> MERLWKDIKRDWLLYAMLLPTIIWFLIFLYKPMIGLQMAFKQYSAWKGIAGSPWIGFDHFVTLFQSEQFIRAIKNTLTLSGLSLLFGFPMPILLALMINEVYSKGYRKAVQTIVYLPHFISIVIVAGLVVTFLSPSTGVVNNMLSWIGLDRVYFLTQPEWFRPIYISSNIWKEAGFDSIVYLAAIMSINPALYESAQVDGATRWQMITRITLPCIVPTIAVLLVIRLGHILE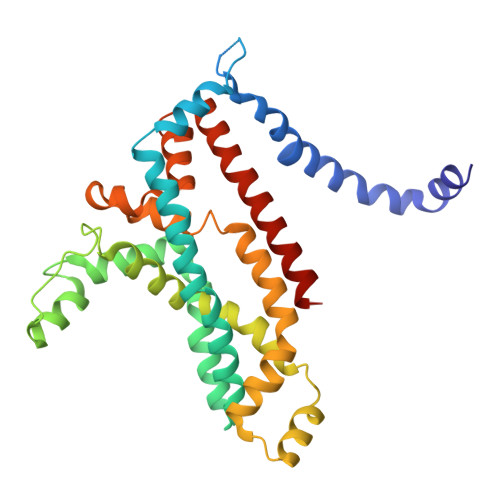VGFEYIILLYQPTTYETADVISTYIYRLGLQGARYDIATAAGIFNAVVALVIVLFANHMSRRITKTGVF>[2x]MHPGFFTSIGQMTDLIHTEKDLVTSLKDYIKAEEDKLEQIKKWAEKLDRLTSTATKDPEGFVGHPVNAFKLMKRLNTEWSELENL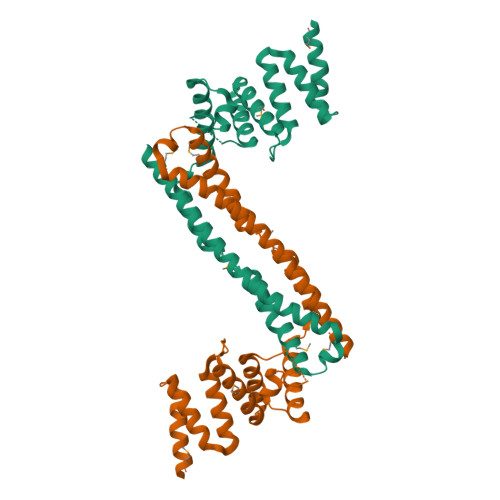VLKDMSDGFISNLTIQRQYFPNDEDQVGAAKALLRLQDTYNLDTDTISKGNLPGVKHKSFLTAEDCFELGKVAYTEADYYHTELWMEQALRQLDEGEISTIDKVSVLDYLSYAVYQQGDLDKALLLTKKLLELDPEHQRANGNLKYFEYIMAKE>MTP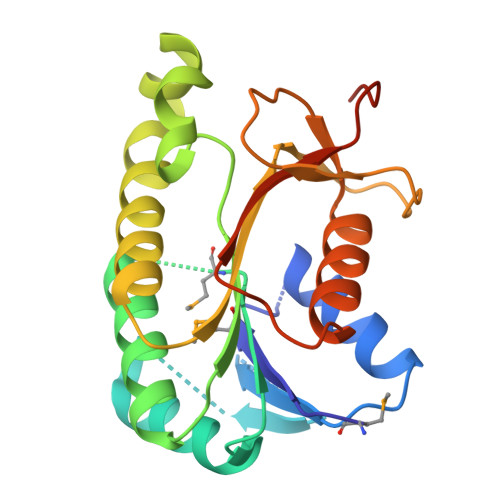WLLFGAGGKGVGARTLELALAEQRPVVAVIRHADAATKLAQQGVQVFTGDACDASVVAAACRAAGPDALIISTMGGAQDYLAHRTVIDEAEKAGITRMILVTSLGCGDSWPFLSERAKAAFGQAVREKTLAESWLQTSQLDYAILRPGGLLDGAATGKAQRIQNQECHGFINRADVAAHIHELANAPALNQQVYSLIEPDLKPALEHHHHHH[2x]>MRPSVSELELSQCDREPIHLLGGIQAYGVLLAFRGPDRRLEVVSANTQALLGRPPEALLGKTAAQVLPAELWAQWELLSARGALRVALPSGPYRALLHESDGLTVLELEPAELQPDMEETALELVRRLVSPLAGAKGTRELLQTAANTVRALTGFDRVMVYRFDADWHGEVLAESKREGMDGFLGMHFPATDIPVQARALYTRNPLRLIANARARPVPLVPSVVPELGRPLDLSGSALRSVSPIHLEYLRNMGVEASFSLSLLKDGALWGLIACHHLAPLHLSYERRRACEVLTQLLALQLSSEERAAEAAEDSHRAALLGPLATSLGAGGTLEEALAKDGARVLELTGATGAALLLGGEPLLVGRTPSMDEVEALAAWLAPQPFQTSFHTERLGSLYPPLAARADVAAGLLAVRLAPASSRLALWFRPEAVRTISWAGNPRKPAEPEPGHARLHPRGSFQAWEETVRETSPAWKRADLAAAEGFRSALIGVVLRQAAELERLSEALSRSNAELDAFGHTVAHDLKEPLRGIQQYAGFVMEDYHGALGPEGRGHMESLMWLA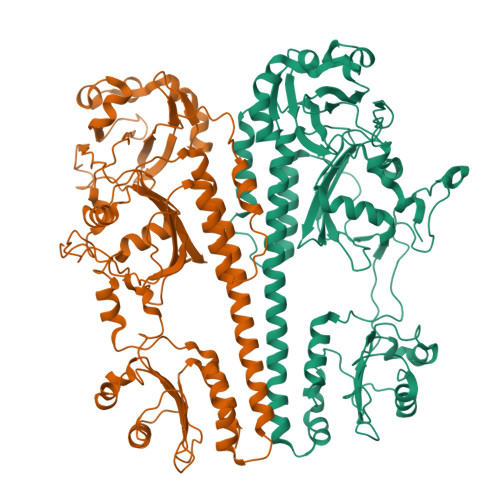QRSGDMLDGLFEYSRAGRVDLAWGEVNMQEVVDEVLATLSTRFQAEKLTVRMPRRLPTVRCDGIRIAQVWANLLVNAAKYQEGPERWVEAGFHGPGEPRPGAAGRYASAYVFYVKDPGIGIAPPFHEAIFEMFRRLHSAKAYGGGTGVGLAIARRLVQLHGGALWVDSAPKQGATFYFTLGRGPG[2x]> MKMTSIQQRAELHRQIWQIANDVRGSVDGWDFKQYVLGALFYRFISENFSSYIEAGDDSICYAKLDDSVITDDIKDDAIKTKGYFIYPSQLFCNV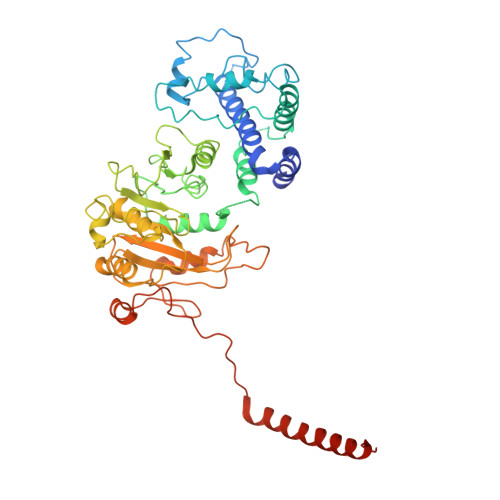AAKANTNDRLNADLNSIFVAIESSAYGYPSEADIKGLFADFDTTSNRLGNTVKDKNARLAAVLKGVEGLKLGDFNEHQIDLFGDAYEFLISNYAANAGKSGGEFFTPQHVSKLIAQLAMHGQTHVNKIYDPAAGSGSLLLQAKKQFDNHIIEEGFFGQEINHTTYNLARMNMFLHNINYDKFDIKLGNTLTEPHFRDEKPFDAIVSNPPYSVKWIGSDDPTLINDERFAPAGVLAPKSKADFAFVLHALNYLSAKGRAAIVCFPGIFYRGGAEQKIRQYLVDNNYVETVISLAPNLFFGTTIAVNILVLSKHKTDTNVQFIDASELFKKETNNNILTDAHIEQIMQVFASKEDVAHLAKSVAFETVVANDYNLSVSSYVEAKDNREIIDIAELNAELKTTVSKIDQLRKDIDAIVAEIEGCEVQK>GSMRTRVRARVISHALKDILAEGDKVIIMGHKRPDLDAIGAAIGVSRFAMMNNLEAYIVLNETDIDPTLRRVMNEIDKKPELRERFITSDDAWDMMTSKTTVVIVDTHKPELVLDENVLNKANRKVVIDHHRRGESFISNPLLIYMEPYASSTAELVTELLEYQPTEQRLTRLESTVMYAGIIVDTRNFTLRTGSRTFDAASYLRAHGADTILTQHFLKDDVDTYINRSELIRTVKVEDNGIAIAHGSDDKIYHPVTVAQAADELLSLEGIEASYVVARREDNLIGISARSLGSVNVQLTMEAL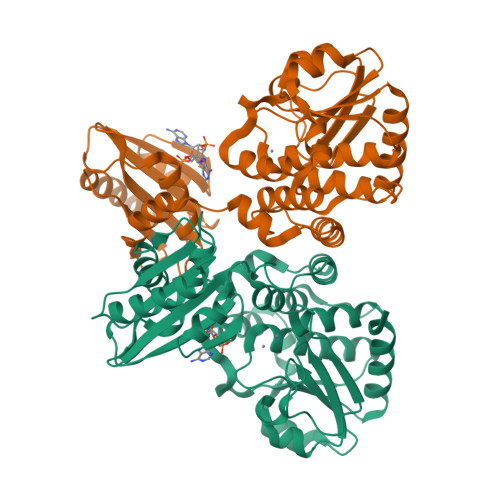GGGGHLTNAATQLKGVTVEEAIAQLQQAITEQLSRSEDA[2x]> MSEKPAESAAAVADSATTTAPQSGKPETALPALIDTQATAETRALYRNLAKLRYKHLLFGHEDSLAYGVHWEGDMDRSDVRDVTGANPAVYGWELGGLELGHTANLDA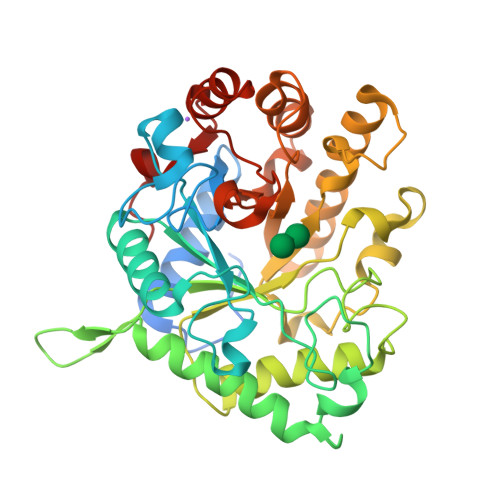VNFEKMQHWIKAGYSRGGVITISWHVFNPVSGGNSWDKTPAVHELIPGGARHATLKAYLDTFVAFNEGLADVDAQGNKHYPPIIFRPWHEHNGDWFWWGKGHASEQDYIALWRFTVHYLRDEKKLRNLIYAYSPDRSRIDMANFEAGYLYGYPGDAYVDIIGLDNYWDVGHEANTASADEQKAALTASLKQLVQIARSKGKIAALTATGNNRLTIDNFWTERLLGPISADADASEIAYVMVWRNANLAREKSEQFFAPFPGQATADDFKRFYQSEVVLFEDELPPLYR> AD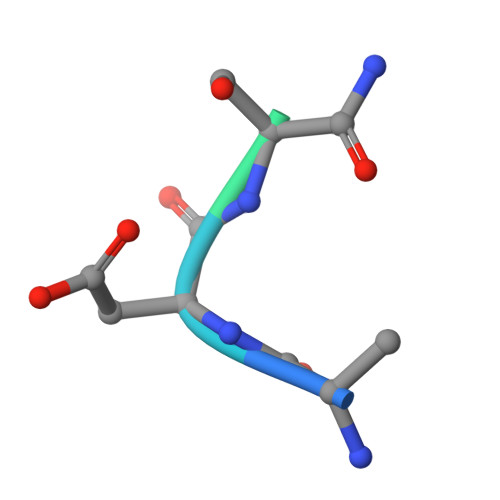SNPIRPVT> SHMQCIVNACKNSWDKSYLAGTPNKDNCSGFVQSVAAELGVPMPRGNANAMVDGLEQSWTKLASGAEAAQKAAQGFLVIAGLKGRTYGHVAVVISGPLYRQKYPMCWCGSIAGAVGQSQGLKSVGQVWNRTDRDRLNYYV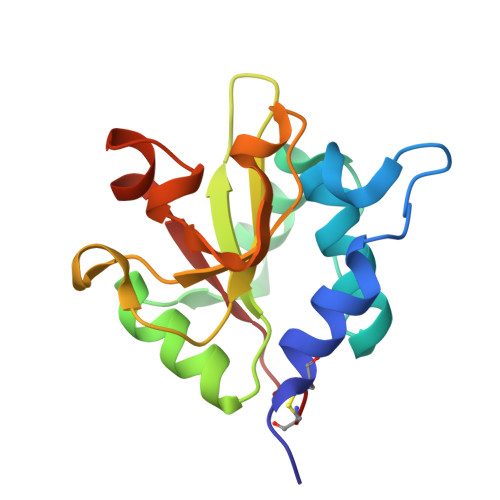YSLASC(2S)-tert-butoxy[7-(8-fluoro-5-methyl-3,4-dihydro-2H-1-benzopyran-6-yl)-5-methyl-2-phenylpyrazolo[1,5-a]pyrimidin-6-yl]acetic 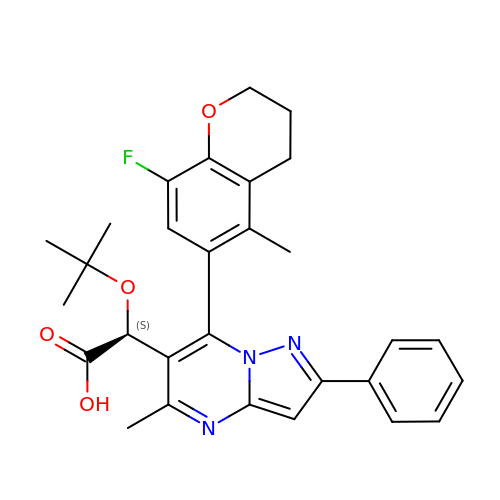acid | C29 H30 F N3 O4 | TZXRURYHFBZSGH-MHZLTWQESA-N> MGFEDGFYTILHLAEGQHPNSKIPGGMYASSKDGKDVPVT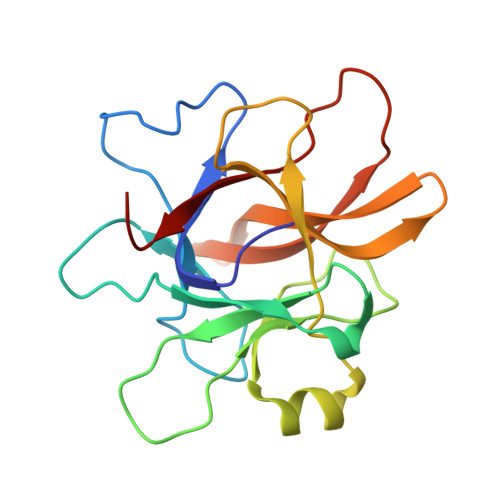AEPLGPQSKIRWWIARDPQAGDDMYTITEFRIDNSIPGQWSRSPVETEVPVYLYDRIKAEETGYTCAWRIQPADHGADGVYHIVGNVRIGSTDWADLREEYGEPQVYMKPVPVIPNVYIPRWFILGYEE>[2x]MVRVAINGFGRIGRLVMRIALSRPNVEVVALNDPFITNDYAAYMFKYDSTHGRYAGEVSHDDKHIIVDGKKIATYQERDPANLPWGSSNVDIAIDSTGVFKELDTAQKHIDAGAKKVVITAPSSTAPMFVMGVNEEKYTSDLKIVSNASCTTNCLAPLAKVINDAFGIEEGLMTTVHSLTATQ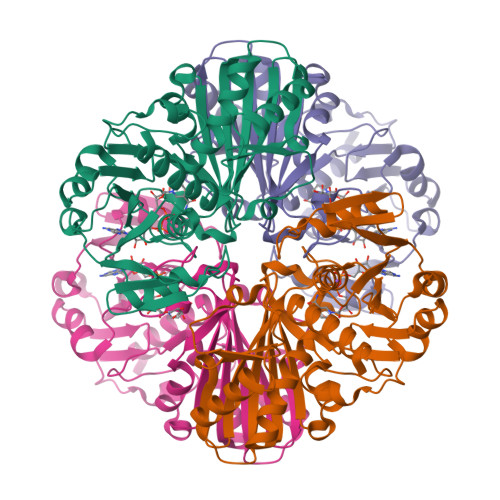KTVDGPSHKDWRGGRTASGNIIPSSTGAAKAVGKVLPELQGKLTGMAFRVPTVDVSVVDLTVKLNKETTYDEIKKVVKAAAEGKLKGVLGYTEDAVVSSDFLGDSHSSIFDASAGIQLSPKFVKLVSWYDNEYGYSTRVVDLVEHVAKA> HDVLETI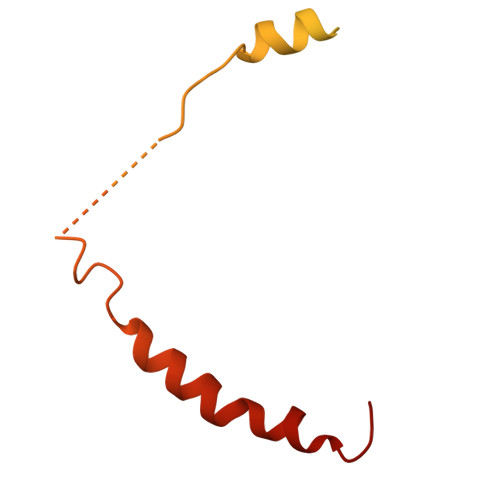FVRKVGAFVNKPINQVTLTSLDIPFAMFAPKNLELEDTDPMVNPPDSPETESPLQGSLHSDGSSGGSSGNTHDDFVMIDFKPAFSKDDILPMDLGTFYREFQNPPQLSSLSIDIGAQSMAEDLDSLPEKLAVHEKNVREFDAFVETLQ> ATSDSNMLLNYVPVYVMLPLGVVNVDNVFEDPDGLKEQLLQLRAAGVDGVMVDVRWGIIELKGPKQYDWRAYRSLFQLVQECGLTLQAIMSFHQCGGNVGDIVNIPIPQWVLDIGESNHDIFYTNRSGTRNKEYLTVGVDNEPIFHGRTAIEIYSDYMKSFRENMSDFLESGLIIDIEVGLGPAGELRYPSYPQSQGWEFPGIGEFQCYDKYLKADFKAAVARAGHPEWELPDDAGKYNDVPESTGFFKSNGTYVTEKGKFFLTWYSNKLLNHGDQILDEANKAFLGCKVKLAIKVSGIHWWYKVENHAAELTAGYYNLNDRDGYRPIARMLSRHHAILNFTCLEMRDSEQPSDAKSGPQELVQQVLSGGWREDIRVAGENALPRYDATAYNQIILNARPQGVNNNGPPKLSMFGVTYLRLSDDL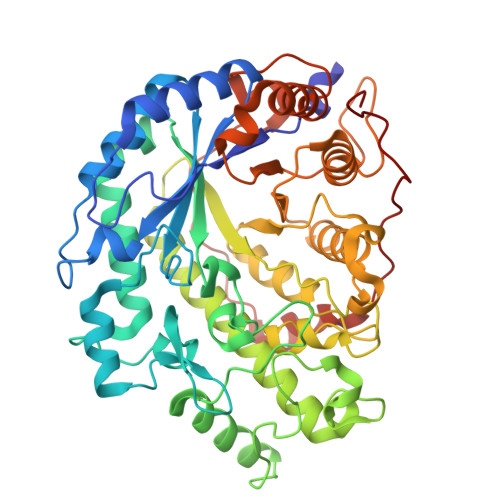LQKSNFNIFKKFVLKMHADQDYCANPQKYNHAITPLKPSAPKIPIEVLLEATKPTLPFPWLPETDMKVDG>GPGSMERRELTYKICLIGDGGVGKTTYINRVLDGRFEKNYNATVGAVNHPVTFLDD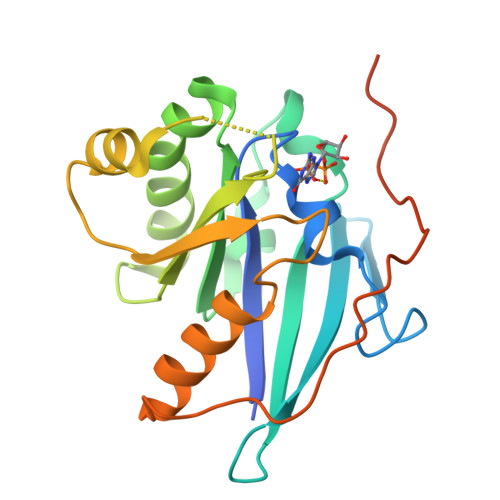QGNVIKFNVWDTAGQEKKAVLKDVYYIGASGAILFFDVTSRITCQNLARWVKEFQAVVGNEAPIVVCANKIDIKNRQKISKKLVMEVLKGKNYEYFEISAKTAHNFGLPFLHLARIFTGRPDLIFVSNVNLEPTEVNYDYHSPEESKYIDYMEQASKMAPEE[2x]> NEQLAKQKGCMACHDLKAKKVGPAYADVAKKYAGRKDAVDYLAGKIKKGGSGVWGSVPMPPQNVTDAEAKQLAQWILSIK

Hydrogenobacter thermophilus (HT) cyt c552 is a thermostable c-type cytochrome. Its high thermostability is achieved by the dense packing of the side chains of hydrophobic amino acids. HT cyt c552 has been shown to form dimers by domain swapping, but the swapping region (N-terminal α-helix and heme) was different from that of horse cyt c12. In this study, we expressed thermostable HT cyt c552 in E. coli cells, and found that HT cyt c552 forms oligomers by domain swapping in E. coli cells.

To investigate formation of oligomers in E. coli, we freeze-thawed E. coli cells expressing wild-type (WT) HT cyt c552, and performed size exclusion chromatography for the extracted solution. Therefore, we attributed the peak at 50–75 ml to HT cyt c552 oligomers. However, no oligomers were detected in the chromatogram when HT cyt c552 and cyt c552 free E. coli lysate were freeze-thawed together, indicating that HT cyt c552 oligomers were formed in E. coli by non-covalent association of its monomers. There was one HT cyt c552 protomer in the asymmetric unit of the crystal, and a domain-swapped structure of dimeric HT cyt c552 was obtained at 1.8 Å resolution. The hinge loop was composed of Ala18, Lys19, and Lys20. The N-terminal α-helix from Asn1 to Lys17, together with the heme, was swapped between protomers in the dimer. The domain-swapped dimer of HT cyt c552 also exhibited high thermostability by maintaining the high density of the amino acid side chains as in the monomer, where the dimer did not dissociate to monomers at 70 °C12. When a holo protein is formed, it creates a transient oligomer with an apo protein. A heme is inserted to the apo protein of the transient holo-apo complex, refolding to a domain-swapped dimer. Our results reveal that more domain-swapped oligomers are formed for more stable proteins, and exceedingly stable proteins may have disadvantages by forming oligomer by-products in cells.>SMYVIRDEWGNQIWICPGCNKPDDGSPMIGCDDCDDWYHWPCVGIMTAPPEEMQWFCPKCANK[2x];>ART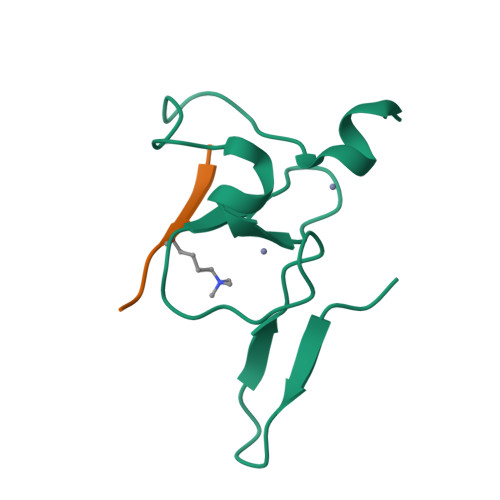KQTA[2x]> MAKREPIHDNSIRTEWE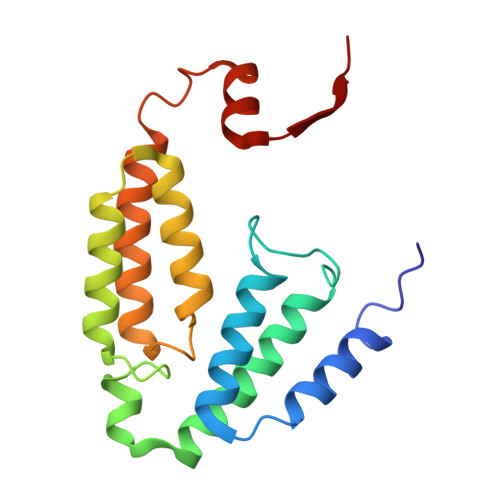AKIAKLTSVDQATKFIQDFRLAYTSPFRKSYDIDVDYQYIERKIEEKLSVLKTEKLPVADLITKATTGEDAAAVEATWIAKIKAAKSKYEAERIHIEFRQLYKPPVLPVNVFLRTDAALGTVLMEIRNTDYYGTPLEGLRKERGVKVLHLQA On the other hand, the CASTOR1 homodimer and the CASTOR1-CASTOR2 heterodimer function as a cytosolic arginine sensor, and negatively regulate mTORC1 activity by binding to and inhibiting GATOR2. In the absence of arginine, CASTOR1 binds to GATOR2 and inhibits mTORC1 signaling; whereas in the presence of arginine, CASTOR1 interacts with arginine and no longer associates with GATOR2. Both CASTOR1 and CASTOR2 were found to contain two putative Aspartate kinase, Chorismate mutase, and TyrA (ACT) domains which function to recognize small ligands such as amino acids and nucleotides. In this study, we determined the crystal structure of human CASTOR1 in complex with a tightly bound arginine.

By using the single-wavelength anomalous dispersion (SAD) method with a selenomethionine (SeMet) derivative, we determined the crystal structure of full-length human CATSOR1 in complex with arginine to 2.07 Å resolution, with the Rwork/Rfree factors being 19.00%/23.83%. In the crystal structure, CASTOR1 forms a dimer with the two protomers related by a two-fold rotation axis, and each protomer contains a bound arginine. Dimerization buries ~935 Å2 of surface area for each protomer, and is mainly mediated through juxtaposition of the α1 and α5 helices of CASTOR1. Yet, our structure shows that each protomer of CASTOR1 actually contains four, rather than the proposed two, ACT domains. ACT1 (residues 1–75) and ACT2 (residues 76–153) assemble into the N-terminal domain (NTD, residues 1–153), while ACT3 (residues 175–260) and ACT4 (residues 261–329) form the C-terminal domain (CTD, residues 175–329). The NTD and CTD are reminiscent of two halves of a sphere, and the bound arginine molecule is encased inside this sphere. The arginine molecule is completely buried inside CASTOR1, and is located at the interface between CASTOR1-NTD and -CTD. The side-chain carboxyl group of Asp304 and the main-chain carbonyl groups of Gly274, Thr300, Phe301, and Phe303, all from CASTOR1-CTD, form charge-stabilized hydrogen bonds with the guanidinium group of arginine. In addition, the side-chain hydroxyl group of Ser111 and the main-chain carbonyl group of Val112, both from CASTOR1-NTD, accept hydrogen bonds from the main-chain amino group of arginine. Besides, the main-chain amino group of Ile280 and the main-chain carbonyl group of Glu277, both from CASTOR1-CTD, make hydrogen bonds with the main-chain carboxyl group of arginine.

>MGSHHHHHHSSGLVPRGSHMELHILEHRVRVLSVARPGLWLYTHPLIKLLFLPRRSRCKFFSLTETPEDYTLMVDEEGFKELPPSEFLQVAEATWLVLNVSSHSGAAVQAAGVTKIARSVIAPLAEHHVSVLMLSTYQTDFILVREQDLSVVIHTLAQEFDIYREVGGEPVPVTRDDSSNGFPRTQHGPSPTVHPIQSPQNRFCVLTLDPETLPAIATTLIDVLFYSHSTPKEAASSSPEPSSITFFAFSLIEGYISIVMDAETQKKFPSDLLLTSSSGELWRMVRIGGQPLGFDECGIVAQIAGPLAAADISAYYISTFNFDHALVPEDGIGSVIEVLQRRQEGLASR[2x]> EC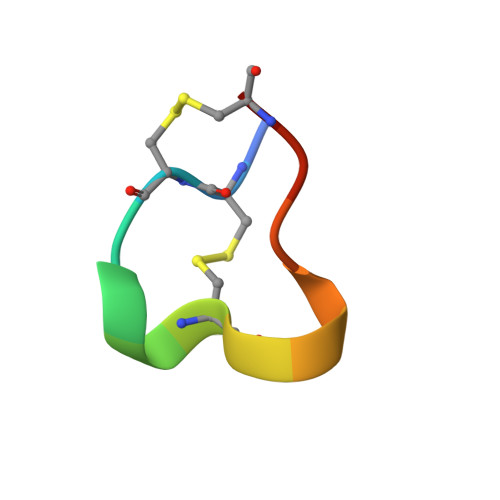CNPACGRHYSCX> MAWKDCIIQRYKDGDVNNIYTANRNEEITIEEYKVFVNEACHPYPVILPDRSVLSGDFTSAYADDDESCYRHHH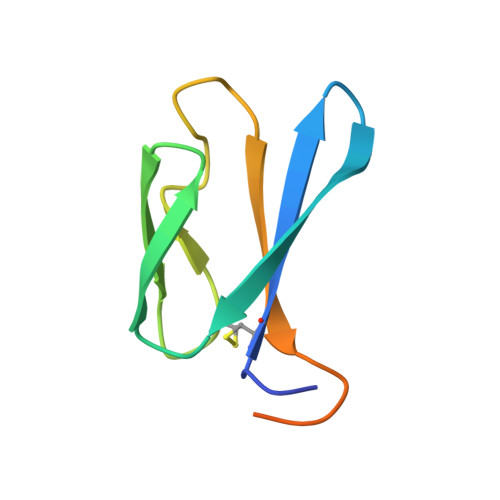HHH> GPLGSFKIYQQKSFEQKIESLKKEKDDQLSEGNQKEHFRQGQAEVIAYYPLQGEKVISSVRELINQDVKDKLESKDNLVFYYTEQEESGLKGVVNRNVTK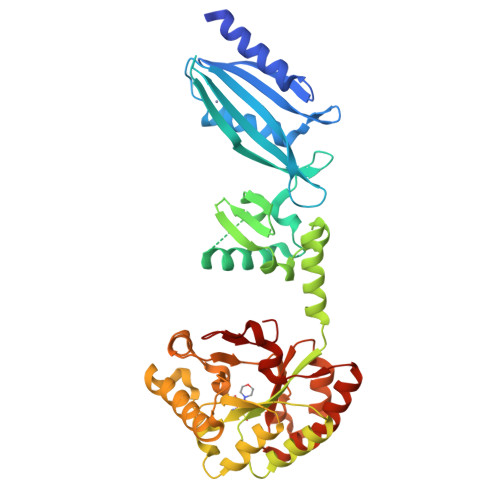QIYDLVAFKIEETEKTSLGKVHLTEDGQPFTLDQLFSDASKAKEQLIKELTSFIEDKKIEQDQSEQIVKNFSDQDLSAWNFDYKDSQIILYPSPVVENLEEIALPVSAFFDVIQSSYLLEKDAALYQSYFDKKHQKVVALTFNDGPNPATTPQVLETLAKYDIKATFFVLGKNVSGNEDLVKRIKSEGHVVGNHSWSHPILSQLSLDEAKKQITDTEDVLTKVLGSSSKLMRPPYGAITDDIRNSLDLSFIMWDVDSLDWKSKNEASILTEIQHQVANGSIVLMHDIHSPTVNALPRVIEYLKNQGYTFVTIPEMLNTRLKAHELYYSRDE>MKYVVVSGGVISGIGKGVLASSTGMLMKTLGLKVTSIKIDPYMNIDAGTMSPLEHGECFVLDDGGETDLDLGNYERYLGVTLTKDHNITTGKIYSHVIAKERKGDYLGKTVQIVPHLTNAIQDWIERVAKIPVDDTGMEPDVCIIELGGTVGDIESAPFVEALRQFQFKVGKENFALIHVSLVPVIHGEQKTKPTQAAIKGLRSLGLVPDMIACRCSETLDKPTIDKIAMFCHVGPEQVVNVHDVNSTYHVPLLLLEQKMIDYLHARLKLDEISLTEEEELLSKWKATTGNFDETVKIALVGKYTNLKDSYLSVIKALEHSSMKCRRKLDIKWVEATDLEPEAQESNKTKFHEAWNMVSTADGILIPGGFGVRGTEGMVLAARWARENHIPFLGVCLGLQIATIEFTRSVLGRKDSHSAEFYPDIDEKNHVVVFMMRLGLRPTFFQNETEWSQIKKLYGDVSEVHERHRHRYEINPKMVDELENNGLIFVGKDDTGKRCEILELKNHPYYIATQYHPEYTSKVLDPSKPFLGLVAASAGILQDVIEGKYDLEA[12x]

CTP synthase (CTPS) catalyzes the final, rate-limiting step of de novo CTP biosynthesis (Lieberman, 1956). Each CTPS monomer consists of a glutaminase domain and an amido-ligase domain connected by an alpha helical linker. Glutamine hydrolysis in the glutaminase domain produces ammonia which is transferred through a channel into the amido-ligase domain, where it is ligated to UTP to form CTP in an ATP-dependent process. Budding yeast have two CTPS isoforms, Ura7 and Ura8, which share 78 % identical residues.

We solved filament structures of both Ura7 and Ura8 in substrate- (ATP and UTP) and product- (CTP) bound states. Ura7 filaments reached lower resolutions, 7.3 Å (substrates) and 3.7 Å (products), but the overall structures were indistinguishable from Ura8 at these resolutions. Like other previously reported structures of human, Drosophila, and E. coli CTPS, the yeast enzyme assembles as stacked tetramers. However, it does so using a completely different interaction interface, which was the same in both substrate- and product-bound yeast structures. Helix 356–370 in the glutaminase domain mediates interactions between tetramers, so that each protomer is involved in assembly contacts. Residues painted similar (yellow) and different (red) from Ura8. In addition, Ura7 assembles with the W363/W392 hydrophobic core shown in Figure 3. Indeed, the major source of heterogeneity in single Ura7-substrate filaments, which were flexible and short, are tetramers that only make one contact at each paired assembly interface. This leads to tetramers in the active, substrate-bound conformation tethered to each other through single glutaminase domain interactions. Thus, filament assembly with symmetric contacts acts as a steric constraint to trap yeast CTPS in a low activity conformation, while tethering through a single glutaminase domain supports short, flexible filaments that accommodate a fully active conformation.>EIKTTTTLHRVVEETTKPLGATLVVETDISRKDVNGLARGHLVDGIPLCTPSFYADIAMQVGQYSMQRLRAGHPGAGAIDGLVDVSDMVVDKALVPHGKGPQLLRTTLTMEWPPKAAATTRSAKVKFATYFADGKLDTEHASCTVRFTSDAQLKSLRRSVSEYKTHIRQLHDGHAKGQFMRYNRKTGYKLMSSMARFNP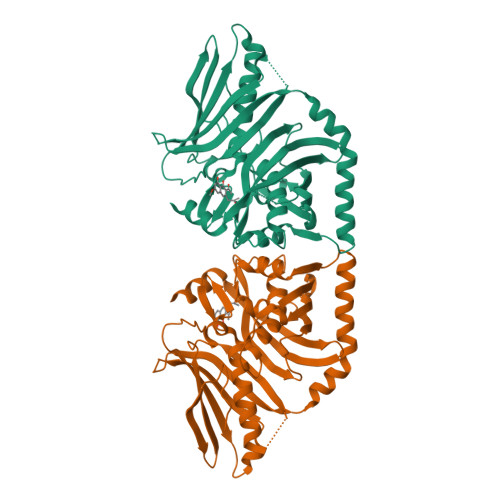DYMLLDYLVLNEAENEAASGVDFSLGSSEGTFAAHPAHVDAITQVAGFAMNANDNVDIEKQVYVNHGWDSFQIYQPLDNSKSYQVYTKMGQAKENDLVHGDVVVLDGEQIVAFFRGLTLRSVPRGALRVVLQTTVKKADRQLGFKTMPSPPPPTTTM[2x]> GAGCAGACATG;> ACTGCACTCA;> CAAGT;> TCTGAGTGCTG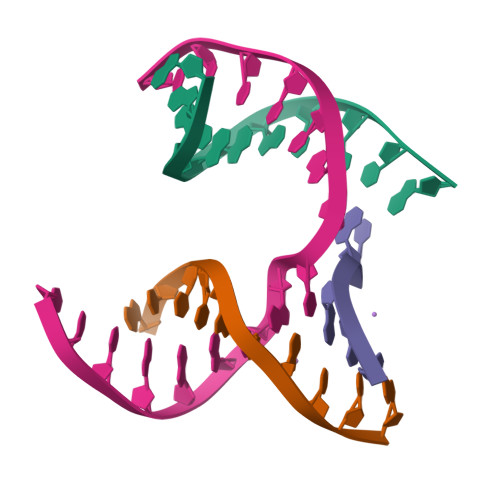TCTGC>MASQTITVGPWGGPGGNEWDDGSYTGIRIIELSYKEAIGSFSVIYDLNGEPFSGSKHTSKLPYTNVKIELQFPEEFLVSVSGYTAPFSSLATRTPVVRSLKFKTNKGRTFGPYGEEDGTYFNLPIENGLVVGFKGRTGDLLDAIGVHMAL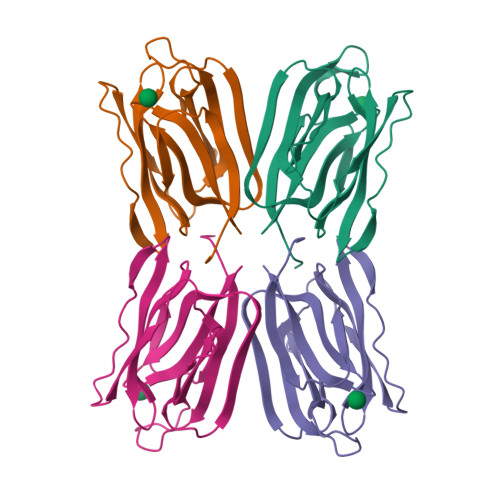[4x]> PR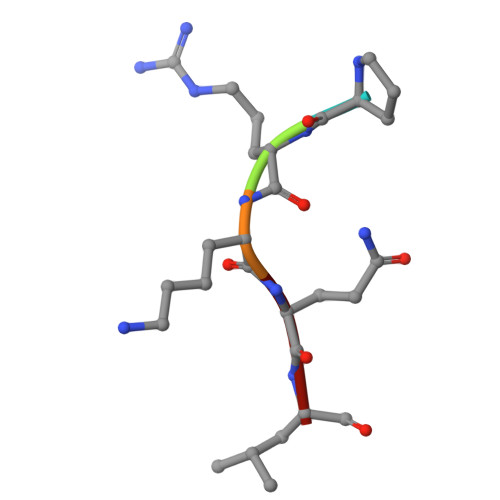KQL>DSYYQRSDWTADEEQILLGPFDYLESLPGKNMRSQLIQSFNTWLKVPTESLDVIIKVISMLHTASLLIDDIQDQSILRRGQPVAHSIFGTAQAMNSGNYVYFLALREVQKLQNPKAISIYVDSLIDLARGQGMELFWRDSLMCPTEEQYLDMVANKTGGLFCLAIQLMQAEATIQVDFIPLVRLLGIIFQICDDYLNLKSTAYTDNKGLCEDLTEGKFSFPIIHSIRSNPGNRQLINILKQKPREDDIKRYALSYMESTNSFEYTRGVVRKLKTEAIDTIQGLEKHGLEENIGIRKILARMSLEL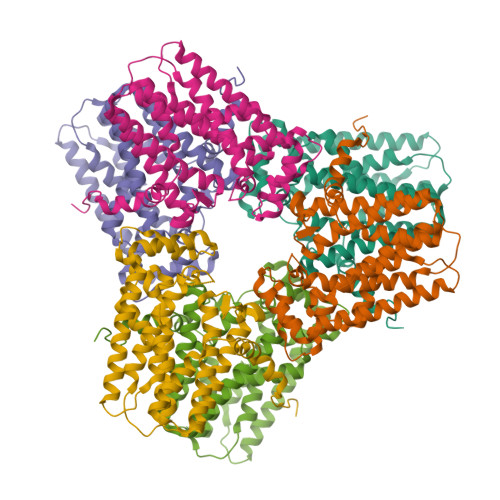[2x]>[4x]VKLAGNSSLCPVSGWAIYSKDNSVRIGSKGDVFVIREPFISCSPLECRTFFLTQGALLNDK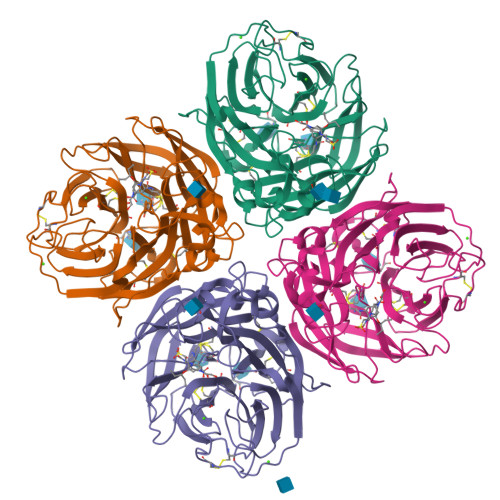HSNGTIKDRSPYRTLMSCPIGEVPSPYNSRFESVAWSASACHDGINWLTIGISGPDNGAVAVLKYNGIITDTIKSWRNNILRTQESECACVNGSCFTVMTDGPSNGQASYKIFRIEKGKIVKSVEMNAPNYHYEECSCYPDSSEITCVCRDNWHGSNRPWVSFNQNLEYQIGYICSGIFGDNPRPNDKTGSCGPVSSNGANGVKGFSFKYGNGVWIGRTKSISSRNGFEMIWDPNGWTGTDNNFSIKQDIVGINEWSGYSGSFVQHPELTGLDCIRPCFWVELIRGRPKENTIWTSGSSISFCGVNSDTVGWSWPDGAELPFTIDK> MFDIGFSELLLVFIIGLVVLGPQRLPVAVKTVAGWIRALRSLATTVQNELTQELKLQEFQDSLKKVEKASLTNLTPELKASMDELRQAAESMKRSYVANDPEKASDE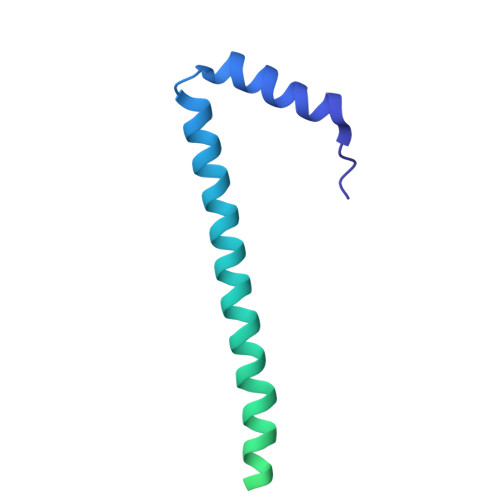AHTIHNPVVKDNEAAHEGVTPAAAQTQASSPEQKPETTPEPVVKPAADAEPKTAAPSPSSSDKP>GAMDPREVILCKDQDGKIGLRLKSIDNGIFVQLVQANSPASLVGLRFGDQVLQINGENCAGWSSDKAHKVLKQAFGEKITMTIRDRPFERTITMHKDSTGHVGFIFKNGKITSIVKDSSAARNGLLTEHNICEI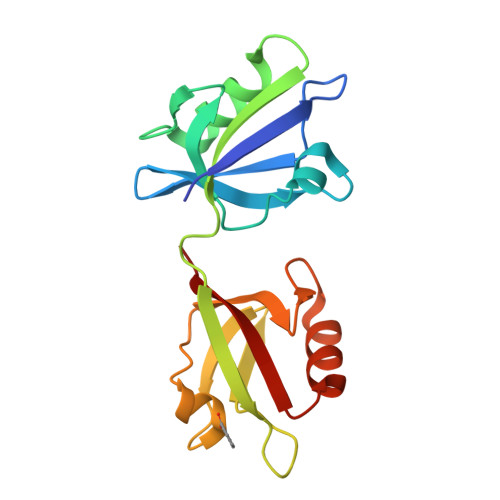NGQNVIGLKDSQIADILSTSGTVVTITIMPAF[2x];> TNEFAF> MGTYEIRGQVASGFGDQSWDASSFAGFYYDIDDNVSTETLTVSDLDGNVIPEGGLVYTTTIADVDFEYYNPDAGWDQYPVMGFFAEEYIPINPDKADKIAKLVLDSDDKYTIRTGEMLDLGEGYAIEAKQ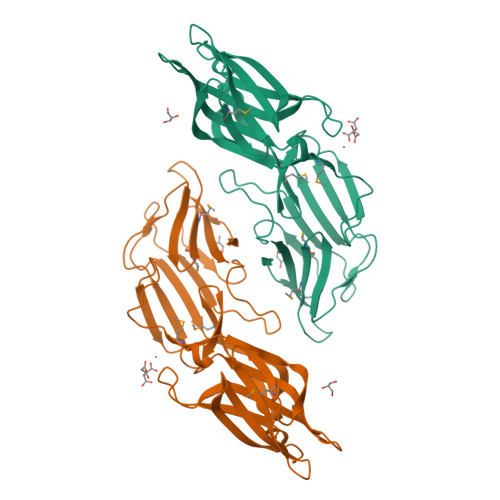VDVDGEKVWLEFTKDGEFVDDEIISVSTADDEANTWDVELDDIEDEDDVVVLKVHVNQVFQGAVDSIAQIEGLWLIDYANAMTIESDDEFGNLDDVSIDGDTLKISNEDTFTLTRDSEEEIGEGMYFMIADTSSSDLRYYPYVEKTIGLEHHHHHH SULFOQUINOVOSE-URIDINE-C1,5'-DIPHOSPHATE | C15 H24 N2 O19 P2 S | 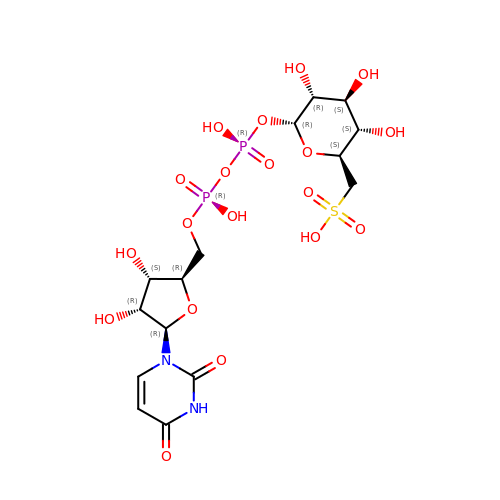FQANCGQCBCUSMI-JZMIEXBBSA-N6-fluoroanthraniloyl-AMP | C17 H18 F N6 O8 P | 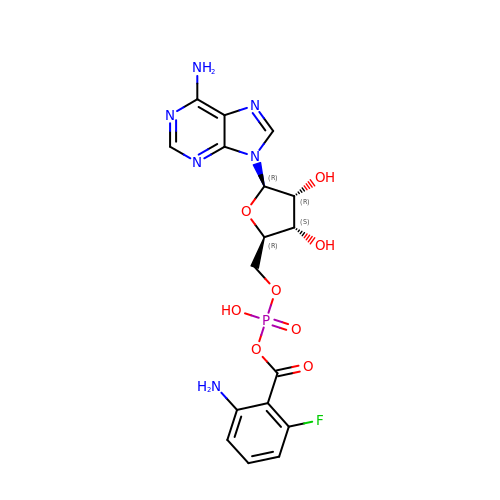IWRUVECWXLGDCT-RVXWVPLUSA-N> HHHHHHGSMGFLILSRREGEGITLSLKADYPAEELIRQLREGGIRILVTDIIGNQARVGIEAPRGVLIVRDELKTAPKG

In bacteria, the highly conserved RsmA/CsrA family of RNA-binding proteins functions as global posttranscriptional regulators acting on mRNA translation and stability. Through phenotypic complementation of an rsmA mutant in Pseudomonas aeruginosa, we discovered a family member, termed RsmN. Elucidation of the RsmN crystal structure and that of the complex with a hairpin from the sRNA, RsmZ, reveals a uniquely inserted α helix, which redirects the polypeptide chain to form a distinctly different protein fold to the domain-swapped dimeric structure of RsmA homologs. The overall β sheet structure required for RNA recognition is, however, preserved with compensatory sequence and structure differences, allowing the RsmN dimer to target binding motifs in both structured hairpin loops and flexible disordered RNAs.

We have solved the crystal structure of RsmN at 2.0 Å resolution and report a distinctly different polypeptide fold to the domain-swapped dimeric structure described for RsmA homologs (Gutiérrez et al., 2005; Heeb et al., 2006; Schubert et al., 2007). The asymmetric unit contains a single RsmN molecule, with the electron density allowing model building of the first 66 residues from RsmN out of a total of 71. The RsmN structure is distinct and completely novel compared with those of all other RsmA/CsrA orthologs and reveals that the 16-residue insert between β strands 2 and 3 has the effect of redirecting the polypeptide chain to give a unique dimer structure. The RsmN dimer consists of a very similar ten-stranded interface held together by a sandwich of two five-stranded β sheets assembled in the same order: β5-β2-β3-β4-β1. The structure lacks the α helix at the C terminus, but instead, the 16-residue insert adopts a well-defined α helix between β strands 2 and 3, with the sequences represented as β1-β2-α-β3-β4-β5 and β1-β2-β3-β4-β5-α, respectively, for RsmN and RsmA. In RsmN, the noticeable difference is that the insertion of the α helix between β2-β3 sterically prevents these consecutive β strands from lying adjacent and antiparallel to each other within the same sheet. Instead, the α helix forces the polypeptide chain to cross over to form part of the other β sheet, such that the RsmN β sheets are composed as follows: β5A-β2A-β3B-β4B-β1B and β5B-β2B-β3A-β4A-β1A. Thus, the overall folding topology of the two polypeptide chains and their dimerization interface is altered by the presence of the α helical insert, making the dimer interface no longer domain swapped but the product of two docked folded monomers (Figure 3A versus Figure 3B). Surface area analysis shows that RsmA buries at ∼4,453 Å2 in its interwined dimer structure; however, this is significantly smaller for the RsmN dimer (2,841 Å2).>[2x]MAISIKTPEDIEKMRVAGRLAAEVLEMIEPYVKPGVSTGELDRICNDYIVNEQHAVSACLGYHGYPKSVCISINEVVCHGIPDDAKLLKDGDIVNIDVTVIKDGFHGDTSKMFIVGKPTIMGERLCRITQESLYLALRMVKPGINLREIGAAIQKFVEAEGFSVVREYCGHGIGRGFHEEPQVLHYDSRETNVVLKPGMTFTIEPMVNAGKKE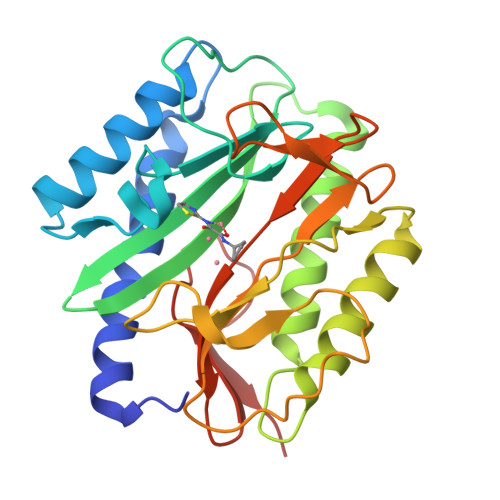IRTMKDGWTVKTKDRSLSAQYEHTIVVTDNGCEILTLRKDDTIPAIISHDE> AVSVAAQKLRLALDMYEVGEQMQRMRLG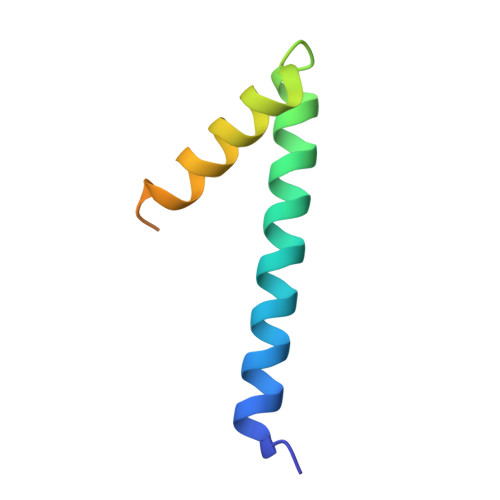RERPNADVVEIEAAIDAWRMTRPGAEEGDSAGPTSTRFT> SGDTDEPIFGKKPRIEESITEDLSLADLMPRVKVQSVETVEGCTHEVALPAEEDYLPLKPRVGKAAKEYPFILDAFQREAIQCVDNNQSVLVSAHTSAGKTVCAEYAIALALREKQRVIFTSPIKALSNQKYREMYEEFQDVGLMTGDVTINPTASCLVMTTEILRSMLYRGSEVMREVAWVIFDEIHYMRDSERGVVWEETIILLPDNVHYVFLSATIPNARQFAEWICHLHKQPCHVIYTDYRPTPLQHYIFPAGGDGLHLVVDENGDFREDNFNTAMQVLRDAGDLAKGDQKGRKGGTKGPSNVFKIVKMIMERNFQPVIIFSFSKKDCEAYALQMTKLDFNTDEEKKMVEEVFSNAIDCLSDEDKKLPQVEHVLPLLKRGIGIHHGGLLPILKETIEILFSEGLIKALFATETFAMGINMPARTVLFTNARKFDGKDFRWISSGEYIQMSGRAGRRGMDDRGIVILMVDEKMSPTIGKQLLKGSADPLNSAFHLTYNMVLNLLRVEEINPEYMLEKSFYQFQHYRAIPGSRTVLQMDELKCRKRVLRRLGFATSSDVIEMKGRVACEISSADELLLTEMMFNGLFNDLSAEQATALLSCFVFQENSSEMPKLTEQLAGPLRQMQECAKRIAKVSAEAKLEIDEETYLSSFKPHLMDVVYTWATGATFAHICKMTDVFEGSIIRCMRRLEELLRQMCQAAKAIGNTELENKFAEGITKIKRDIVFAASLYL;> SGDPIPDMSKFATGITPFEFENMAESTGMYLRIRSL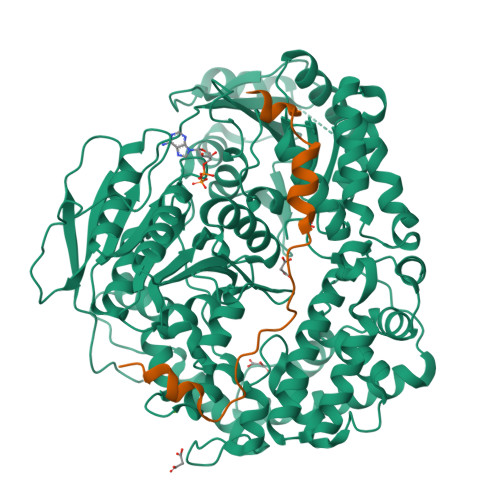LKNSPRNQQKNKKASE METHYL-PHOSPHONIC ACID MONO-(4-NITRO-PHENYL) ESTER 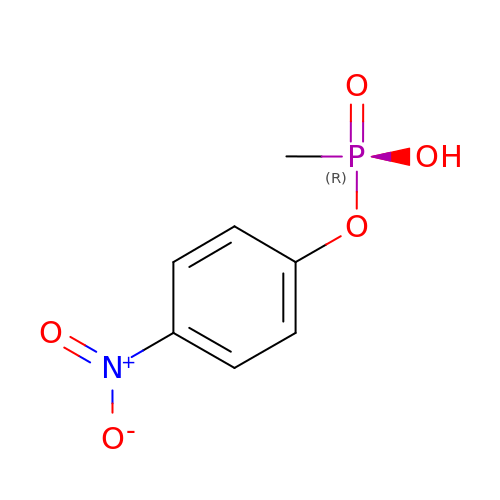| C7 H8 N O5 P | VJPXTXIEAOSJBR-UHFFFAOYSA-N>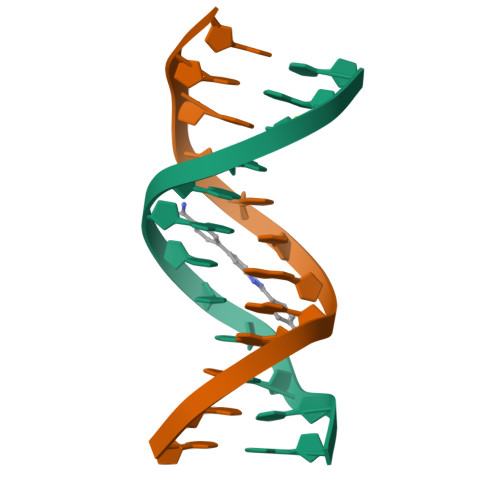CGCGAATTCGCG[2x]> MENS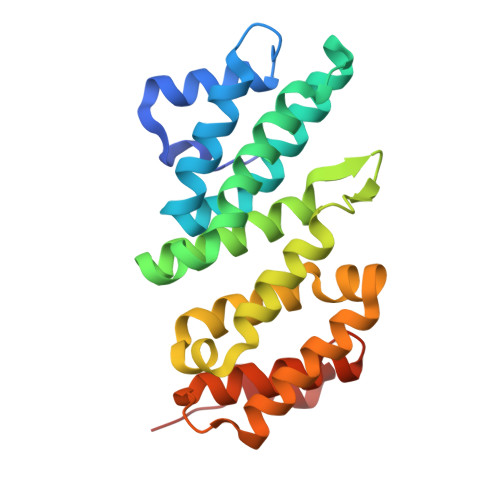SKEDYKIQSFDLETQKLLKTALKDPGSVDLEKVSSVIVDQSLKDQVFSREAGRICYTIVQAEAKQTNGSVFRRNLLNRLQQEFKAREETRKRSTQEWVCLVSFICNIFDYLKVNNMPMVALVHPVYDCLFRLAQSDALKNEEEVDCLVLQLHRIGDQLEKMNVQLMDELFNLLRDGFLLQEDLSSMGRLLLLEILEFRAGGWKLSDTAQKYYYSEVTD> KRNK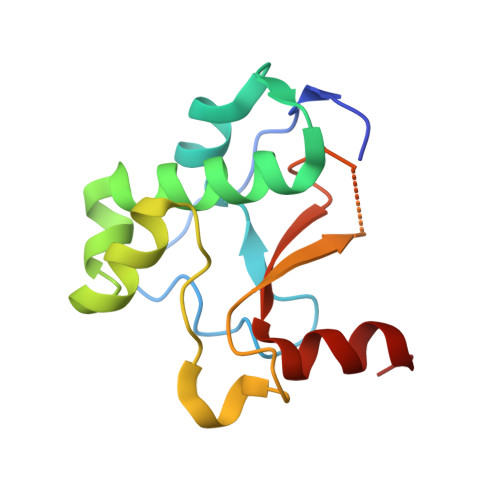PGKATGKGKPVNNKWLNNAGKDLGSPVPDRIANKLRDKEFKSFDDFRKKFWEEVSKDPELSKQFSRNNNDRMKVGKAPKTRTQDVSGKRTSFELHHEKPISQNGGVYDMDAISVVTPKRHIDIHRGK>MSASDALNSCPHVALLLSSGMGHLTPCLRFAATLVQHHCRVTIITNYPTVSVAESRAISLLLSDFPQITEKQFHLLPFDPSTANTTDPFFLRWEAIRRSAHLLNPLLSSISPPLSALVIDSSLVSSFVPVAANLDLPSYVLFTSSTRMCSLEETFPAFVASKTNFDSIQLDDVIEIPGFSPVPVSSVPPVFLNLNHLFTTMLIQNGQSFRKANGILINTFEALEGGILPGINDKRAADGLPPYCSVGPLLPCKFEKTECSAPVKWLDDQPEGSVVYVSFGSRFALSSEQIKELGDGLIRSGCRFLWVVKCKKVDQEDEESLDELLGRDVLEKIK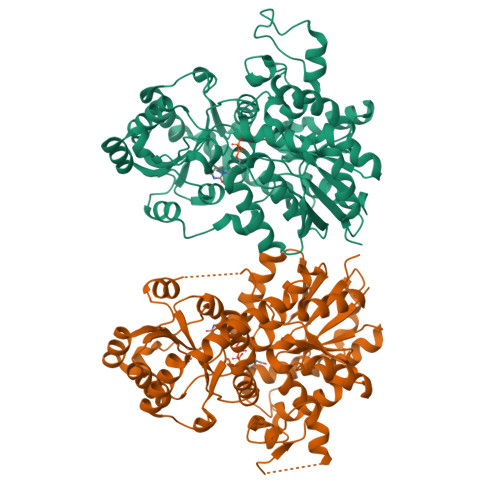KYGFVIKNWVNQQEILDHRAVGGFVTHGGWNSSMEAVWHGVPMLVWPQFGDQKINAEVIERSGLGMWVKRWGWGTQQLVKGEEIGERIKDLMGNNPLRVRAKTLREEARKAIEVGGSSEKTLKELIENWKKTSRKT[2x]> GPLPGKNAPSTAGLGYGSWEIDPKDLTFLKELGTGQFGVVKYGKWRGQYDVAIKMIKEGSMSEDEFIEEAKVMMNLSHEKLVQLYGVCTKQRPIFIITEYMANGCLLNYLREMRHRFQTQQLLEMCKDVCEAMEYLESKQFLHRDLAARNCLVNDQGVVKVSDFGLSRYVLDDEYTSSVGSKFPVRWSPPEVLMYSKFSSKSDIWAFGVLMWEIYSLGKMPYERFTNSETAEHIAQGLRLYRPHLASEKVYT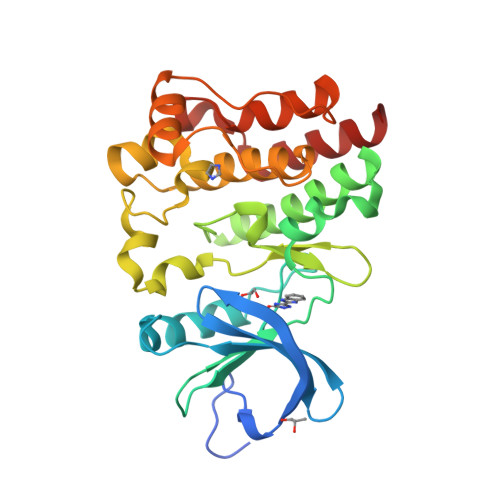IMYSCWHEKADERPTFKILLSNILDVMDEES>[2x]FEFPEELKTKLQEHINYFPKKRQAILLCLHEIQNYYGYIPPESLKPLADMLELPLNHVEGVVAFYDMFDREDKAKYRIRVCVSIVCHLMGTNKLLKALENILGIKPGEVTPDGKFKIVPVQCLGACSEAPVFMVNDDEYKFESEVQLNEILSRYT;>[2x]RSYPAIPRIYAETTLNMLLKRAKKPRVHSIDEYLKDGGYQALEKALNMSPEEIIDWVDKSTLRGRGGAGFPTGKKWKFAVQNPGPRYFICNADEMEPGTFKDRIIIERDPHLLIEGIIISSYAIGANEAYIYIRGEYPAGYYILRDAIEE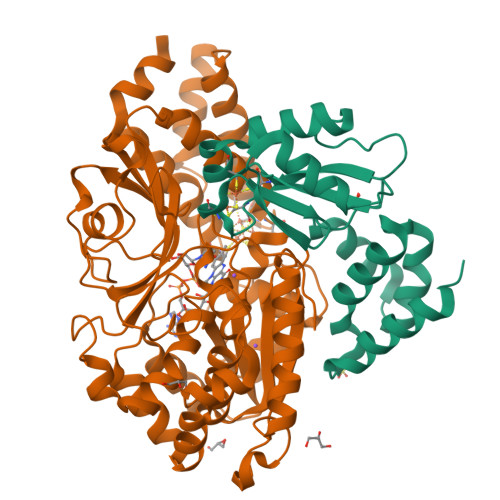AKKKGFLGKNILGSGFDLEIYVARGAGAYICGEETALIESLEGKRGHPRLKPPYPVQKGLWGKPTVVNNVETIANVPFIISMGWEEYRYIGPSDYAGPKLFPVSGKVKKPGVYELPMNTTLREVIFKYAGGTLGNKKVKAVFSGALDCFSSEELDIPMDYSPLGFGGTGTVIVLTEEDDIVEAALKIAEFYEHETCGQCTPCRVGCYEQANLLEKIYKGEATEQDWEGFDFVNRNIQPTSICGLGAVAGRLIRQTLEKFPEEWEKYRK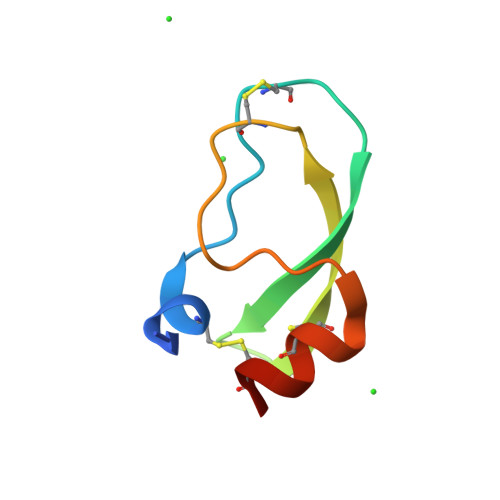> EAEASICSEPKKVGRCKGYFPRFYFDSETGKCTPFIYGGCGGNGNNFETLHQCRAICRLG>PSLPPEIIVISANMSLEDQIKIARETIPIAPGAQTSEELGRLTENLKSFADKTFGGCWQVMVVDGSYWITQTFVPNMSFQ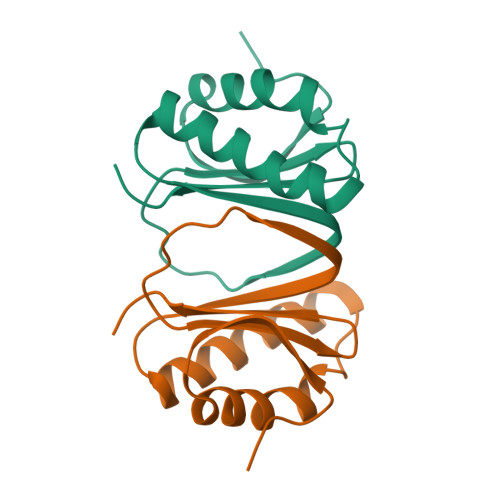FELYNRAYLFWQTSE[3x]> GHMAGVLTENLVLQKTKVDSIQRVRKLNVCAAQLSDIGVLRRACNLEVLSLSLNELSELGVLE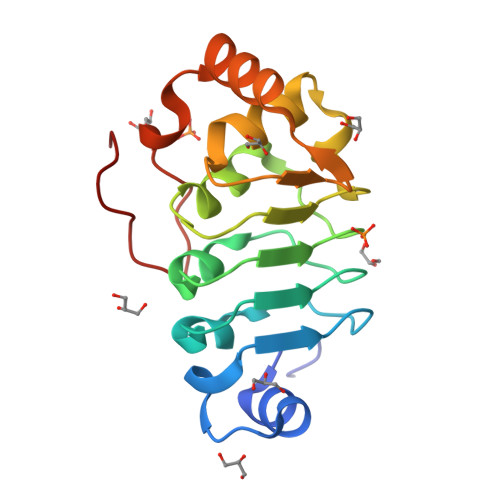NCPRLSELYLRKNRVEDLNQVLHLSDAPNLTVLTLTENPICQDPNYRRFVIAAVGSLQRLDDIDILPQEREEAYRVFPNLHAIAPPPSLYCDPAKGKIR N-{2-[({3-[6-(piperazin-1-yl)pyridin-3-yl]-1H-indazol-5-yl}amino)methyl]phenyl}methanesulfonamide | C24 H27 N7 O2 S | 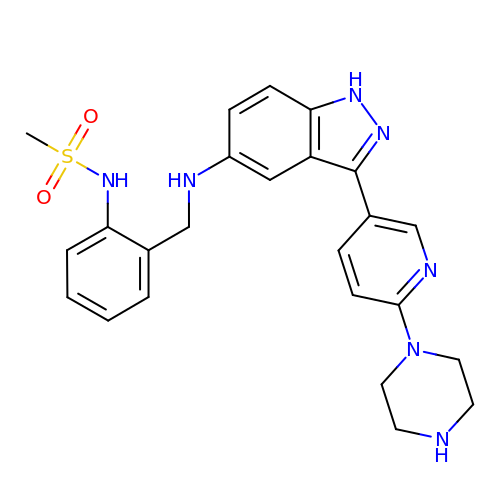ZTJQDVXGJTWIGK-UHFFFAOYSA-N>MLTFALTIVRAGETQYNRDKLLQGQGIDTPLSDTGHQQAAAAGRYLKDLHFTNVFVSNLQRAIQTAEIILGNNLHSSATEMILDPLLRER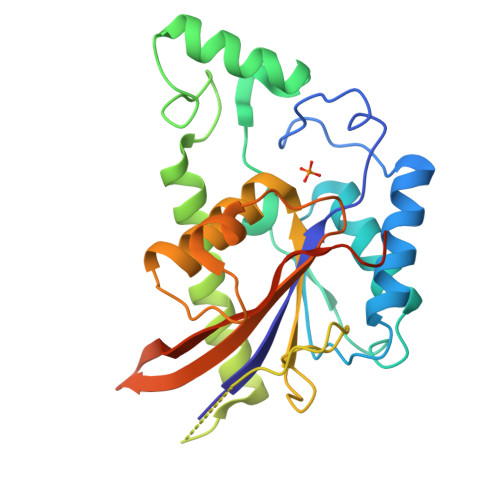GFGVAEGRPKEHLKNMANAAGQSCRDYTPPGGETLEQVKTRFKMFLKSLFQRMFEEHGSALSSVPSEADQPVIAGLADDGAQNVPVHALMVSHGAFIRISVRHLVEDLQCCLPAGLKMNQVFSPCPNTGISRFIFTIHREESVLRATRIQGVFINRKDHLEEVKNSDLEHHHHHH[2x]>[2x]KMNESDIWFEEKLQEVECEEQRLRKLHAVVETLVNHRKELALNTAQFAKSLAMLGSSEDNTALSRALSQLAEVEEKIEQLHQEQANNDFFLLAELLSDYIRLLAIVRAAFDQRMKTWQRWQDAQATLQKKREAEARLLWANKPDKLQQAKDEILEWESRVTQYERDFERISTVVRKEVIRFEKEKSKDFKNHVIKYLETLLYSQQQLAKYWEAFLPEAKAIS;>DEVLFTGVKEVDDFFEQEKNFLINYYNRIKDSCVKADKMTRSHKNVADDYIHTAACLHSLALEEPTVIKKYLLKVAELFEKLRKVEGRVSSDEDLKLTELLRYYMLNIEAAKDLLYRRTKALIDYENSNKALDKARLKSKDVKLAEAHQQECCQKFEQLSESAKEELINFKRKRVAAFRKNLIEMSELEIKHARNNVSLLQSCIDLFKNN[2x]

A key component of the recycling machinery is the endosomal sorting complex for promoting exit 1 (ESCPE-1), which rescues transmembrane proteins from the endolysosomal pathway for transport to the trans-Golgi network and the plasma membrane. The SNX protein family is defined by the presence of a phox-homology (PX) domain that typically binds phosphatidylinositol phospholipids (PtdInsPs), but may also participate in protein–protein interactions. Twelve out of the 33 annotated mammalian SNXs contain an additional carboxy-terminal Bin/Amphiphysin/Rvs (BAR) domain, and are therefore denoted as the PX-BAR or SNX-BAR subfamily. Herein, we show that ESCPE-1 has a single-layer coat organization and suggest how synergistic interactions between ESCPE-1 protomers, phosphoinositides and cargo molecules result in a global arrangement of amphipathic helices to drive tubule formation.

To understand the molecular basis for heterodimerization between ESCPE-1 protomers and its membrane tubulation activity, we determined the crystal structure of SNX1BAR–SNX5BAR (where BAR stands for the BAR domains of both proteins) at 2.5 Å resolution. The structure forms an antiparallel dimer of three-helix bundles with a curvature that would fit a circle with a diameter of ~32 nm. Electron density at the tip of SNX5BAR is very weak, indicating flexibility of this region. Unlike other SNX-BAR homodimers, the SNX1BAR–SNX5BAR heterodimer exhibits asymmetry on its surface properties, general shape, and the associated PX domains located at either side of the BAR heterodimer. The interface buries a large area of 5,114 Å2, of which 78% corresponds to polar surface. From this analysis, we found that two clusters formed by F347 and W511 in SNX1, and F273 and F401 in SNX5, have the highest binding energy. Yet, only F347 and W511 in SNX1 are conserved, indicating that these residues likely form a binding hot spot. SNX1BAR and SNX5BAR exhibit complementary polarity at their distal and proximal interfaces. Consistent with previous predictions, the central region of SNX5BAR has a negative patch, whereas the equivalent region in SNX1BAR is neutral. The crystal structure of the SNX1BAR–SNX5BAR complex presented here, together with analytical modeling, revealed that SNX1 comprises a hydrophobic binding hot spot compatible with homodimerization and heterodimerization, whereas SNX5 uses distinct patches of polar residues to preclude homodimerization and enhance heterodimerization.>[2x]VSFRQKRTRIPLLAMTVTALAAAVCGVTTAPAATGAEVAVPLSVGAAAGNATPIPGYVIQSSAQVSDDSAVSKPGFPTSGWYPVSSRSTVYAGLLQNGKYADPFYSTNMQNVPAAQFSVPWWYRTDLNVDDTSSRTYLDFSGVLSKADVWVNGTKVATKDQVNGAYTRHDLDITAQVHTGVNSVAFKVYPNDPNRDLSMGWIDWAQTPPDQNMGIVRDVLVRRSGAVALRSAHVIQKLNSALDHADLTVKADVRNDSANAVQTTVAGTVAGKPISQTVSLAAKERKTVTFPLVG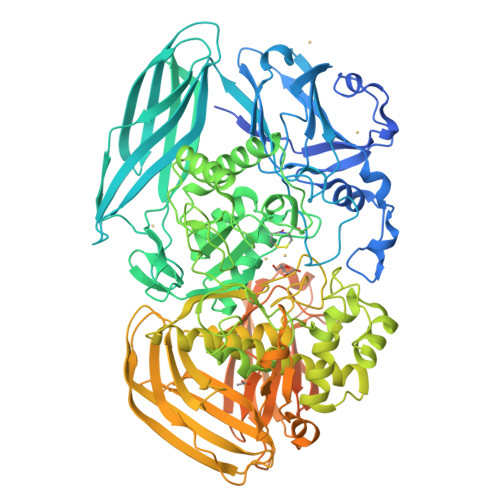LDRPNVWWPAGMGGQHRYDLDLTASVGGTPSDAAKSKFGVRDVKATLNSSGGRQYSVNGKPLLIRGGGYTPDLFLRWNETAAADKLKYVLNLGLNTVRLEGHIEPDEFFDIADDLGVLTMPGWECCDKWEGQVNGEEKGEPWVESDYPIAKASMFSEAERLRDHPSVISFHIGSEFAPDRRIEQGYLDAMKAADFLLPVIPAASARPSPITGASGMKMNGPYDYVPPVYWYDKSQKDRGGAWSFNSETSAGVDIPTMDTLKRMMSASELDTMWKNPSAKQYHRSSSDTFGNLKLFGDALTKRYGASANLNDFVRKAQLSQYENVRAEFESHSRNYTDSTNPSTGLIYWMLNSPWTSLHWQLFDAYMDQNGAYYGAKKANEPLHIQYSHDNRSVVVINQTSNAVSGLTATTKLYNLDGTEKYSNTKTGLSVGALGAKATAVTVPAVSGLSTTYLAKNVLTDSSGKEVSRNVYWLSTKADTLNWGGSDWYYTPQSAFADLSGLNNLGQSAVGATANSVAGADGTTTTTVTLKNTSGGRLPAFYVDSKVVDSAGKPVLPVEWNDNAVSLWPGETTTLTAKYRTADLKGSKPSVRISGWNTGTQTVPADGSGPGPSDPVDYQAEDATIVQGAVESNHAGYTGTGFVNYDNVAGSSVEWTVTVPSAGTYDVVVRYANGTTTSRPLDFSVNGSISASGVAFGSTGTWPAWTTKTVRVTLAAGVNKIKAVATTANGGPNVDKITL>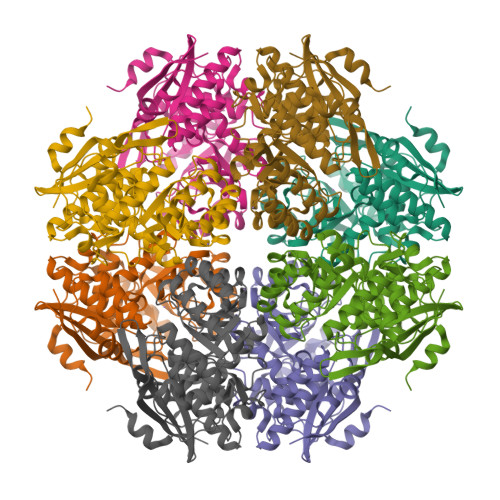 MKIEAISTTIVDVPTRRPLQMSFTTVHKQSYVIVQVKAGGLVGIGEGGSVGGPTWGSESAETIKVIIDNYLAPLLVGKDASNLSQARVLMDRAVTGNLSAKAAIDIALHDLKARALNLSIADLIGGTMRTSIPIAWTLASGDTARDIDSALEMIETRRHNRFKVKLGARTPAQDLEHIRSIVKAVGDRASVRVDVNQGWDEQTASIWIPRLEEAGVELVEQPVPRANFGALRRLTEQNGVAILADESLSSLSSAFELARDHAVDAFSLKLCNMGGIANTLKVAAVAEAAGISSYGGTMLDSTVGTAAALHVYATLPSLPYGCELIGPWVLGDRLTQQDLEIKDFEVHLPLGSGLGVDLDHDKVRHYTRAA>[2x]MAHHHHHHVDDDDKMVHHDGFQTVKATIDWEHPMFKLYEKAKRNGKWNPADIDFSQDQKDFASLTSEEKISALPLVAGFSAGEEAVTLDILPMAHALARQGRLEDVL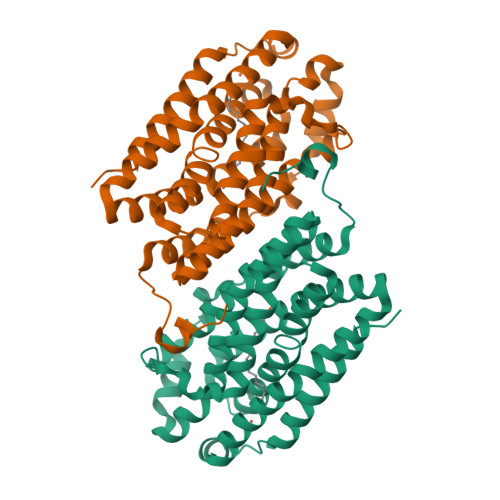FLTTFMHDEAKHVEMFSRWQQAVGIGQMDLSVFHNDHYKRIFYEALPEAMNRLYADDSPEAVIRAATVYNMIVEGTLAESGFYTFRQIYKKAGLFPGLLQGIDYLNMDEGRHIQFGIYTIQRIVNEDERYYELFIRYMDELWPHVIGYVDYLTELGKRQQQLARTYALEIDYDLLRHYVIKQFNLRKKQISRTKRVDVVEGLEKTAAES Compared to the RdRPs of other Flaviviridae representatives such as the NS5 of the Japanese encephalitis virus (JEV) and dengue virus (DENV) in the Flavivirus genus and the NS5B of the hepatitis C virus (HCV) of the Hepacivirus genus, the pestivirus NS5B contains a unique ∼90-residue N-terminal domain (NTD) that does not have notable sequence homology to any other viral or host proteins. The global conformation of our CSFV NS5B structures is consistent with the recently reported CSFV structure with an RMSD value of 0.9 Å (95% coverage) between the reported structure and our representative C-682 structure. These structures together reveal that the NTD adopts a globular α/β fold with an α-β-α-β-β-α pattern. The NTD interacts with the palm of the RdRP core intra-molecularly with a mixture of hydrophobic and hydrogen bonding interactions. Collectively, these biochemical data indicated that the RNA synthesis fidelity of CSFV NS5B is fine-tuned by its NTD through the intra-molecular interactions with the RdRP palm.

In contrast, deletion of residue 673–694 (construct C-672) in the C-terminal tail resulted in apparent reduction of product level (compare lanes 2 and 4). Further truncations beyond residue 681 led to apparent reduction of product level (compare lanes 10–13 to lane 6), suggesting that the N-terminal half (residues 665–680) of the C-terminal tail is likely required for optimal de novo synthesis. The structures of the C-682 and C-672 were solved at 2.1 and 2.3 Å resolution, respectively, in the same crystal form by molecular replacement using the structure of the WT as the search model. These three structures, each containing one NS5B molecule in the crystallographic asymmetric unit, are highly similar with root mean square deviation (RMSD) values of 0.4–0.6 Å between the WT and two C-terminal truncation mutants for all superimposable α-carbon atoms with 99% coverage of the resolved residues in the structure of the WT. Therefore, all three structures are not sufficient to provide a structural basis for why residues up to residue 680 are essential for the de novo-mode synthesis, but are valid for assessing the NTD–RdRP interactions described as follows. Different from the observations in the WT BVDV, full-length JEV, HCV and the recently reported CSFV RdRP structures that have a canonical fold optimal for NTP entry and binding, the CSFV NS5B ring finger bent toward the pinky finger, partially occupying the template RNA binding channel. In the chromatography analysis, the crystallographic open conformation C-672_AA and the C-672, or the AA mutant and the WT, had consistent retention volumes.

> MSNWVMQEENKQGNLTPLFEELLQQCPPGGQNKTAHMVSAYQLAQGNWMPTSCHVFMGTISARRTKTHPYEAYVKLRELVEEHKMKTLCPGSSLGKHNDWIIGKIKYQGNLRTKHMLNPGKVAEQLCREGHRHNVYNKTIGSVMTATGIRLEKLPVVRAQTDTTNFHQAIRDKIDKEENLQTPGLHKKLMEVFNALKRPELESSYDAVEWEELERGINRKGAAGFFERKNIGEILDSEKNKVEEIIDNLKKGRNIKYYETAIPKNEKRDVNDDWTAGDFVDEKKPRVIQYPEAKTRLAITKVMYKWVKQKPVVIPGYEGKTPLFQIFDKVKKEWDQFQNPVAVSFDTKAWDTQVTTKDLELIKDIQKYYFKKKWHKFIDTLTMHMTEVPVICADGEVYIRKGQRGSGQPDTSAGNSMLNVLTMVYAFCEATGVPYKSFDRVAKIHVCGDDGFLITERALGEKFASKGVQILYEAGKPQKITEGDKMKVAYQFDDIEFCSHTPIQVRWSDNTSSYMPGRNTTTILAKMATRLDSSGERGTIAYEKAVAFSFLLMYSWNPLIRRICLLVLSTELQVKPGKSTTYYYEGDPISAYKEVIGHNLFDLKRTSFEKLAKLNLSMSVLGAWTRHTSKRLLQDCVNMGVKEGNWLVNADRLVSSKTGNRYIPGEGHTLQGRGSSSHHHHHH> MAGNDSNLIWLDLEMTGLEPVEDVILEIAIIITDSELNILAQGPIFAISQTDDVLDNMNPWCIEHHGKSGLTQRCRDSEVSLAHATKESLAFVQEWVPQGKSPMCGNSIGQDRRFINKYMPDFEDHFHYRNLDVSTIKELAKRWKPEVLESVVKTGAHLALDDIKESIAELKVYRELFFKL

Therefore, oligoribonucleases (ORN), RNases targeted toward short oligonucleotides, are needed for the complete digestion of short oligonucleotides into mononucleotides. Among these, ORN belongs to the DEDD superfamily, comprising 3′-5′ exonucleases that require a divalent cation for activity. Our research group have focused on the mechanism of action of oligoribonuclease (CpsORN) from the psychrophilic gram-negative bacterium Colwellia psychrerythraea strain 34H, to understand how the enzyme hydrolyses small nucleic acids. Structural analysis results show that CpsORN is a stable dimer and its active site is formed by swapping residues from the other subunit.

The crystal structure of unliganded CpsORN contains five antiparallel β-strands and eight α-helices, with a compact α/β fold. The overall structure of CpsORN was similar to other reported exoribonucleases of the DEDD superfamily. CpsORN has a characteristic core sequence, comprising four invariant acidic amino acids (Asp12, Glu14, Asp112, and Asp163). In the structure of unliganded CpsORN, the α2, α7, α8, and α9 helices, along with the β1 and β2 strands form a negatively charged pocket. A magnesium ion, located in the centre of the pocket, tightly interacts with the invariant acidic amino acids of Asp12, Glu14, Asp112, and Asp163 residues. It should be noted that the unliganded and two separated uridine-bound CpsORN structures contain one metal ion and these structures do not have enough space for second metal binding. The crystals of unliganded CpsORN were obtained from 15% (w/v) PEG 3350 and 0.1 M magnesium formate (MCSG I #G10). Matthews coefficient calculations predicted that one molecule is present in the asymmetric unit, with a Matthew coefficient of 2.45 Å3 Da−1 and 49.79% solvent content. The final model had a Rcryst of 23.51% and a Rfree of 29.69%, with a total of 180 amino acid residues and 30 water molecules.8-{[2-methoxy-5-(4-methylpiperazin-1-yl)phenyl]amino}-1-methyl-4,5-dihydro-1H-pyrazolo[4,3-h]quinazoline-3-carboxamide | C23 H28 N8 O2 | 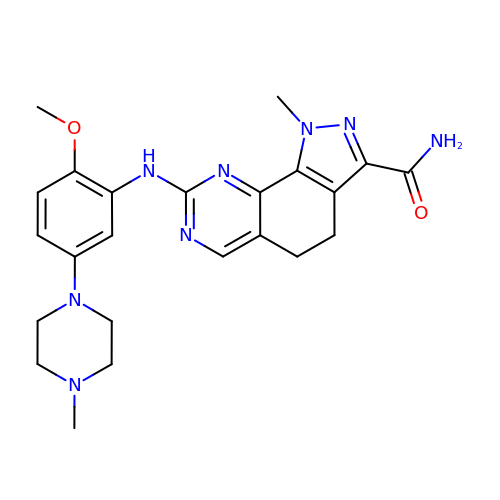SWTRIZHCIUWGAU-UHFFFAOYSA-N>[4x]MNTPEHMTAVVQRFVAALNAGDLDGIVALFADDATVENPVGSEPRSGTAAIREFYANSLKLPLAVELTQEVRAVANEAAFAFIVSFEYQGRKTVVAPIDHFRFNGAGKVVSMRALFGEKNIH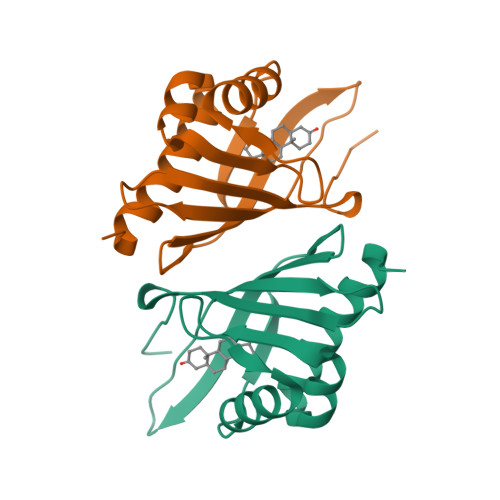AGA>[2x]MMKKADSVPTPAEAALAAQTALAADDSPMGDAARWAMGLLTSSGLPRPEDVAARFIPTFAAAGNFAETVREWRSKGPFTVRAYHPVAHKGWVVLSAPA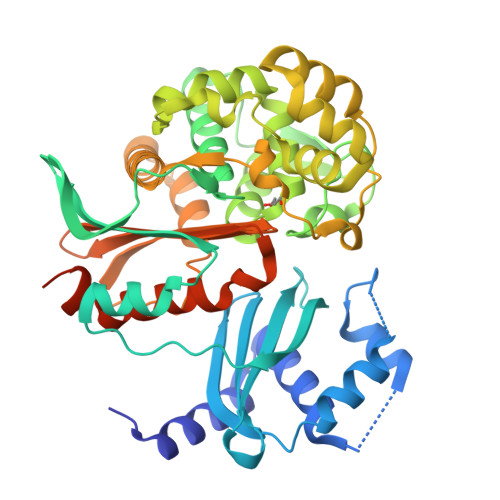GVRYILSLTLDSSGLIRILTLKPETVIPDMVTWNDVEETLHTPGVQHSVYAVRLTPDGHEVLHASAPERPMPTGSAYKLYLMRALVAEIEKGTVGWDEILTLTPELRSLPTGDMQDLPDGTRVTVRETAHKMIALSDNTGADLVADRLGREVVERSLAAAGHHDPSLMRPFLTSHEVFELGWGDPERRAEWVRQDEAGRRELLEKMAGVMTVRGSDLGATVHQLGIDWHMDAFDVVRVLEGLLQDSGRDTSGTVEEILTAYPGLLIDEERWRRVYFKAGASPGVMMFCWLLQDHAGISYVLVLRQSADEQRLIGDGLFLRGIGAKIIEAEAKLLSSGERRGAGTAAAGDDRASAGEAARR> DGGYNAQLAKAKTELNEVSLAIKKSSMKMELLKKELLTIEPKLKEATKDNELNVKHVKQCQETCDKLRARLVEYGFDPSRIKDLKQREDKLKSHYYQTCKNSEYLKRRVTNLEFNYTKPYPNFEASFVHGVVGQLFQIDNDNIRYATALQTCAGGRLFNVVVQDSQTATQLLERGRLRKRVTIIPLDKIYTRPISSQVLDLAKKIAPGKVELAINLIRFDESITKAMEFIFGNSLICEDPETAKKITFHPKIRARSITLQGDVYDPEGTLSGGSRNTSESLLVDIQKYNQIQKQIETIQADLNHVTEELQTQYATSQKTKTIQSDLNLSLHKLDLAKRNLDANPSSQIIARNEEILRDIGECEN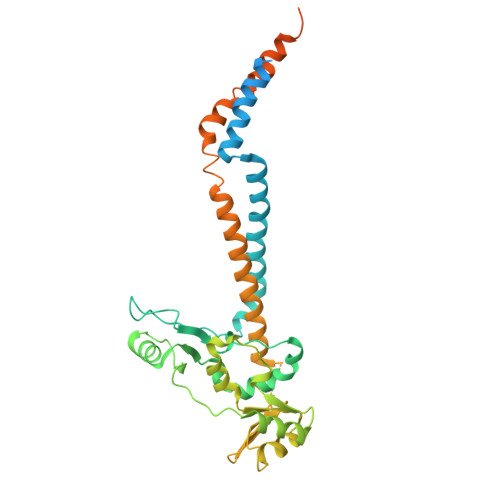EIKTKQMSLKKCQEEVSTIEKDMKEYDSDKGSK> KQGPTSVAYVEVNNNSMLNVGKYTLADGGGNAFDVAVIFAANINYDTGTKTAYLHFNENVQRVLDNAVTQIRPLQQQGIKVLLSVLGNHQGAGFANFPSQQAASAFAKQLSDAVAKYGLDGVDFDDDYAEYGNNGTAQPNDSSFVHLVTALRANMPDKIISLYNIGPAASRLSYGGVDVSDKFDY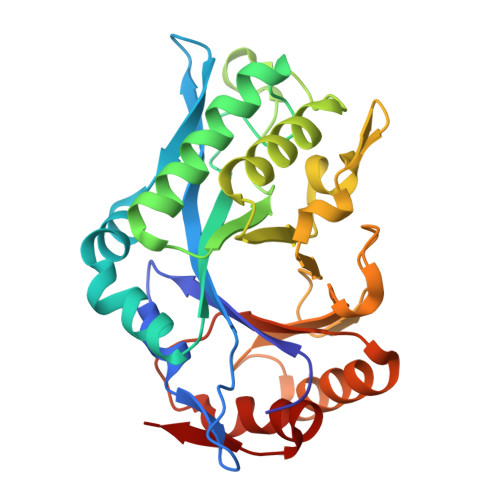AWNPYYGTWQVPGIALPKAQLSPAAVEIGRTSRSTVADLARRTVDEGYGVYLTYNLDGGDRTADVSAFTRELYGSEAVRT N~2~-ACETYL-N~5~-({3-HYDROXY-2-METHYL-5-[(PHOSPHONOOXY)METHYL]PYRIDIN-4-YL}METHYL)-L-ORNITHINE 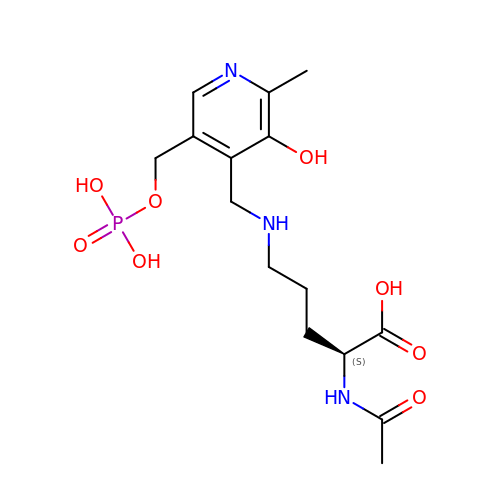| C15 H24 N3 O8 P | QIZZUQLTAZUUFQ-ZDUSSCGKSA-N>[2x]MYLTLQEWN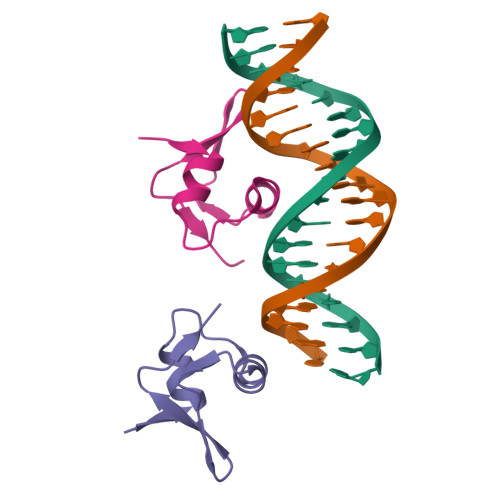ARQRRPRSLETVRRWVRESRIFPPPVKDGREYLFHESAVKVDL>GEVKPRILLMGLRRSGKSSIQKVVFHKMSPNETLFLESTNKICREDVSNSSFVNFQIWDFPGQIDFFDPTFDYEMIFRGTGALIFVIDSQDDYME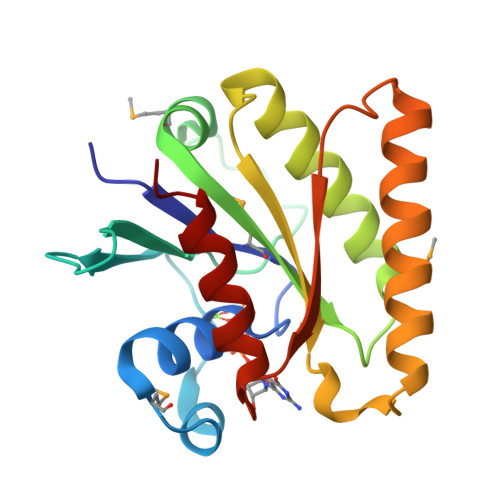ALARLHLTVTRAYKVNTDINFEVFIHKVDGLSDDHKIETQRDIHQRANDDLADAGLEKIHLSFYLTSIYDHSIFEAFSKVVQKLIP[2x]> MASATTSSKNGKPLVVVYGDYKCPYCKELDEKVMPKLRKNYIDNHKVEYQFVNLAFLGKDSIVGSRASHAVLMYAPKSFLDFQKQLFAAQQDE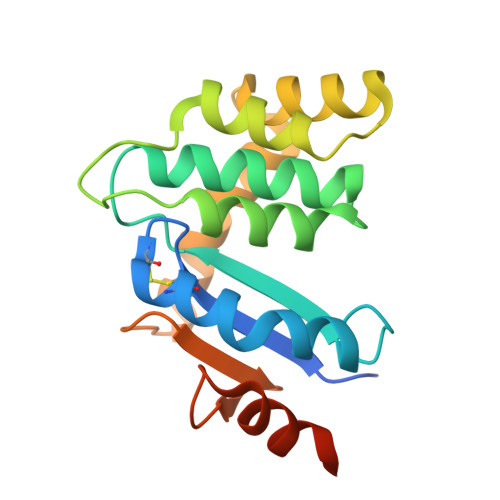NKEWLTKELLDKHIKQLHLDKETENKIIKDYKTKDSKSWKAAEKDKKIAKDNHIKTTPTAFINGEKVEDPYDYESYEKLLKDKIKLEHHHHHH> KPQVTILATGGTIAGVTVDKLLAAVPAINDLATIKGEQISSIGSQEMTGKVWLKLAKRVNELLAQKETEAVIITHGTDTMEETAFFLNLTVKSQKPVVLVGAMRPGSSMSADGPMNLYNAVNVAINKASTNKGVVIVMNDEIHAAREATKLNTTAVNAFASPNTGKIGTVYYGKVE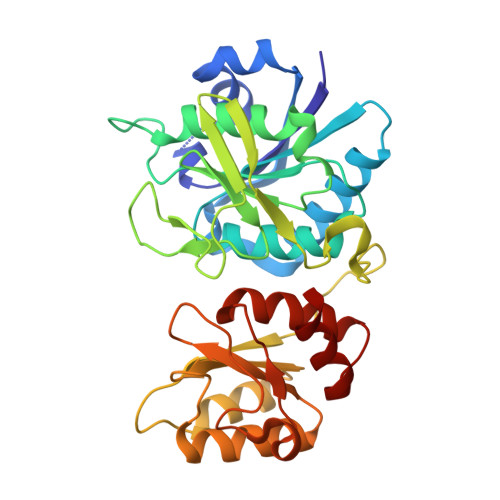YFTQSVRPHTLASEFDISKIEELPRVDILYAHPDDTDVLVNAALQAGAKGIIHAGMGNGNPFPLTQNALEKAAKSGVVVARSSRVGSGSTTQEAEVDDKKLGFVATESLNPQKARVLLMLALTKTSDREAIQKIFSTY>MGAAPDSHQLAKALAEAADVGAQMIKLVGLRELSEAERQLRSLVVALMQEVFTEFFPGCVVHPFGSSINSFDVHGCDLDLFLDLGDLEEPQPVPKLPPASPLLEDREEGDLGKASELAETPKEEKAEGAAMLELVGSILRGCVPGVYRVQTVPSARRPVVKFCHRPSGLHGDVSLSNRLALHNSRFLSLCSELDGRVRPLVYTLRCWAQGRGLSGSGPLLSNYALTLLVIYFLQTRDPPVLPTVSQLTQKAGEGEQVEVDGWDCSFPRDASRLEPSINVEPLSSLLAQFFSAVSSWDLRGSLLSLREGQALPVAGGLPSNLWEGLRLGPLNLQDPFDLSHNVAANVTSRVAGRLQNCCRAAANYCRSLQYQRRSSRGRDWGLLPLLQPSSPSSLLSATPIPLPLAPFTQLTAALVQVFREALGCHIEQATKRTRSEGGGTGQGEAGKGASLPSSASWRCALWHRVWQGRRRARRRLQQQTKEGAGGGAGTRAGWLATEAQVTQELKGLSGGEERPETEPLLSFVASVSPADRMLTVTPLQDPQGLFPDLHHFLQVFLPQAIRHLKLEHHHHHH[4x]

After transcription, the 3′-end is oligo-uridylylated by a terminal uridylyltransferase, TUT1 (TUTase6)910, one of the members of the non-canonical nucleotidyltransferases. TUT1 is composed of N-terminal Zn-finger, RRM, palm, fingers and KA-1 domains. The C-terminal region of TUT1 is a previously unidentified RNA-binding domain, and it was named the KA-1 domain. Thus, the present structural and biochemical studies have demonstrated that TUT1 acts as a U6 snRNA-specific terminal uridylyltransferase.

Therefore, the amino-terminal putative zinc finger (ZF) and RNA recognition motif (RRM) (amino-acid residues 1–140), the predicted disordered proline-rich region (PRR: amino-acid residues 235–304) and the carboxy-terminal region (amino-acid residues 651–750) neighbouring the nuclear localization signal (NLS) were removed. The truncated TUT1 (TUT1_ΔN) was overexpressed in Escherichia coli, purified and crystallized. The form-III crystal belongs to the space group P43212, and its structure was also determined and refined to an R factor of 21.4% (Rfree of 25.8%), using reflections up to 3.4 Å resolution. The form-III TUT1_ΔN adopts a closed conformation, as compared with the form-I TUT1_ΔN. A comparison between the form-I and -III TUT1_ΔN structures highlights the mobility of the KA-1 domain. The KA-1 domain rotates by ∼40° with respect to the catalytic core domains, using α14 as the axis of rotation. The N-terminal RRM is mobile relative to the catalytic core domains, and the C-terminal domain KA-1 domain rotates relative to the catalytic core domains.>HHHHHHMAGMAMDLGGYLTRIGLDGRPRPDLGTLHAIVAAHNRSIPFENLDPLLGIPVADLSAEALFAKLVDRRRGGYCYEHNGLLGYVLEELGFEVERLSGRVVWMRADDAPLPAQTHNVLSVAVPGADGRYLVDVGFGGQTLTSPIRLEAGPVQQTRHEPYRLTRHGDDHTLAAQVRGEWQPLYTFTTEPRPRIDLEVGSWYVSTHPGSHFVTGLTVAVVTDDARYNLRGRNLAVHRSGATEHIRFDSAAQVLDAIVNRFGI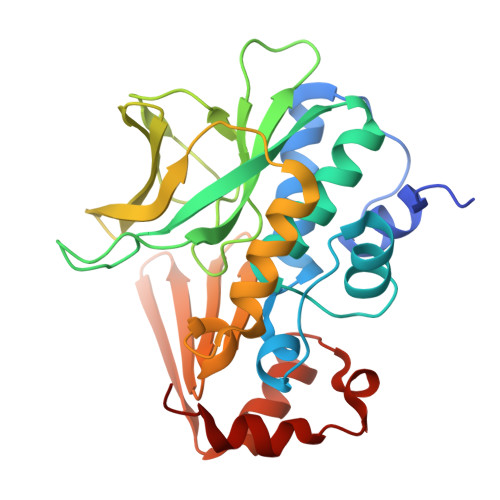DLGDLAGRDVQARVAEVLDT[4x]>MKEKDWWKKSVVYQIYPKSFNDSNGDGVGDIQGIIEKLDYLKELGVDVIWLSPVYDSPQDDNGYDIRDYQKIYEEYGDMATFDQLLQGLHDRDMKLVMDLVVNHTSDEHKWFEESRKSKDNPYRDYYFWREENEINNWGSIFSGPAWELDEKTGEYYLHLFSKKQPDLNWENPKLRQDVYNMMKFWLDKGIDGFRMDVINFISKNTDFPDGPVPDGQIYGDAGNDFCNGPRIHEFLQEMNQEVTSKYDVMTVGEMPGASTTDAQIYTNPANNEVDMIFTFEHMNLDSDSDNKWDLKPIYLPDLKENMSEWQVALQENGWNSLYWNNHDQPRIVSRFGNDNRFRVRSAKMLATCLHMMKGTPYIYQGEEIGMTNVHFETLDDYRDIETLNMYKERKEQGHSHESIMQSIYTKGRDNARTPYQWDNSENAGFTTGTPWLKVNPRYTEINNEEALKNPDSIFYYYQNLIKLRKTTEIITTGNYRLLLPKDEAIFAYERYTENEKLVVLCNFTEEEQVISDETILNEIQKGSV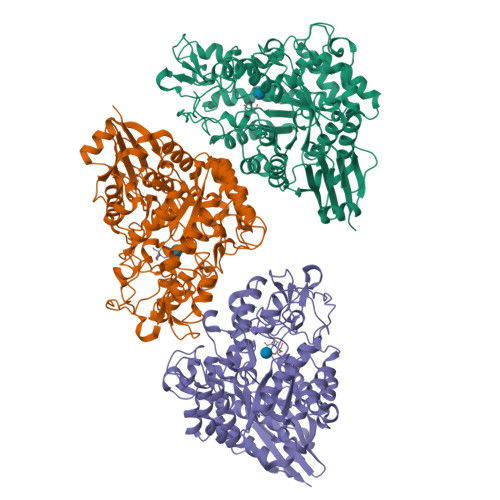LVNNVPNIIEGTLRPYEAIVYQIKGA[3x]> QDADKLPHTKVTLVAPPQVHPHEQATKSGPKVVEFTMTIEEKKMVIDDKGTTLQAMTFNGSMPGPTLVVHEGDYVQLTLVNPATNAMPHNVE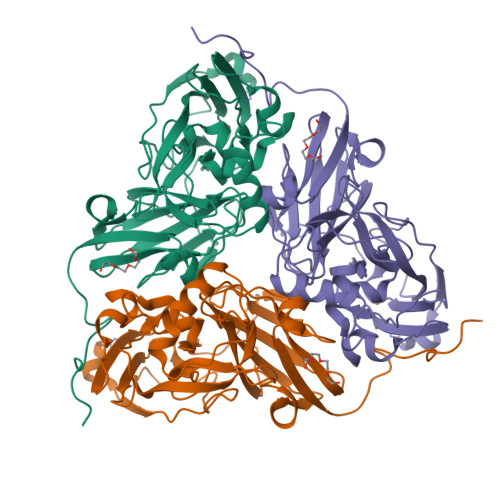FHGATGALGGAKLTNVNPGEQATLRFKADRSGTFVYHCAPEGMVPWHVVSGMSGTLMVLPRDGLKDPQGKPLHYDRAYTIGEFDLYIPKGPDGKYKDYATLAESYGDTVQVMRTLTPSHIVFNGKVGALTGANALTAKVGETVLLIHSQANRDTRPHLIGGHGDWVWETGKFANPPQRDLETWFIRGGSAGAALYTFKQPGVYAYLNHNLIEAFELGAAGHIKVEGKWNDDLMKQIKAPAPIPR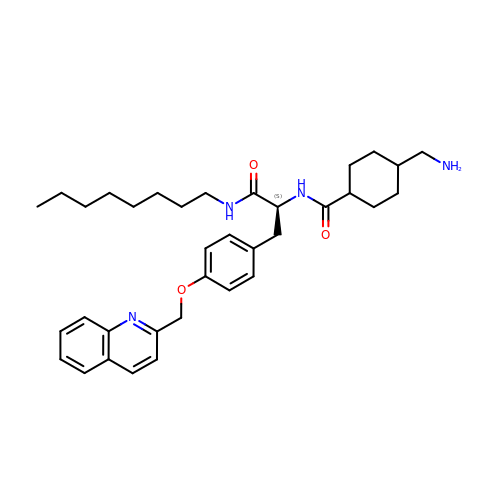Nalpha-[trans-4-(aminomethyl)cyclohexane-1-carbonyl]-N-octyl-O-[(quinolin-2-yl)methyl]-L-tyrosinamide | C35 H48 N4 O3 | ZGUNTZKJIWJKEH-GSZYCOFVSA-N> GSMSSERVLSYAPAFKSFLDTSFFQELSRLKLDVLKLDSTSQPLTVNLDLHNIPKSADQVPLFLTNRSFEKHNNKRTNEVPLQGSIFNFNVLDEFKNLDKQLFLHQRALECWEDGIKDINKCVSFVIISFADLKKYRFYYWLGVPCFQRPSSTVLHVRPEPSLKGLFSKCQKWFDVNYSKWVCILDADDEIVNYDKSIIRKTKVLAIRDTSTMENVPSALTKNFLSVLQYDVPDLIDFKLLIIRQNEGSFALNATFASIDPQSSSSNPDMKVSGWERNVQGKLAPRVVDLSSLLDPLKIADQSVDLNLKLMKWRILPDLNLDIIKNTKVLLLGAGTLGCYVSRALIAWGVRKITFVDNGTVSYSNPVRQALYNFEDAGKPKAELAAASLKRIFPLMDATGVKLSIPMIGHKLVNEEAQHKDFDRLRALIKEHDIIFLLVDSRESRWLPSLLSNIENKTVINAALGFDSYLVMRHGNRDEQSSKQLGCYFCHDVVAPTDSLTDRTLDQMCTVTRPGVAMMASSLAVELMTSLLQTKYSGSETTVLGDIPHQIRGFLHNFSILKLETP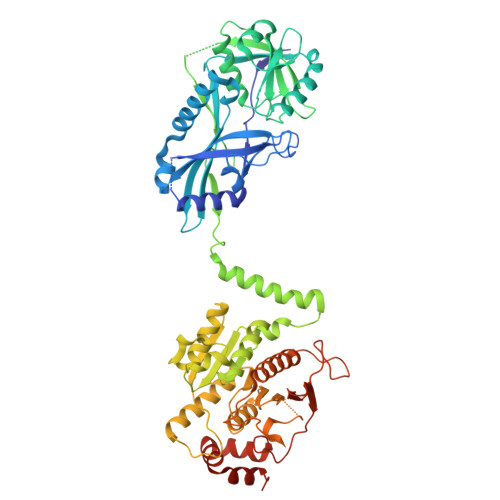AYEHCPACSPKVIEAFTDLGWEFVKKALEHPLYLEEISGLSVIKQEVER During the early and late steps of infection with the Gram-positive bacterium B. anthracis, the tripartite anthrax toxin is secreted as major virulence factor in order to kill host immune cells such as macrophages or neutrophils. Like other AB-type toxins, it is composed of a surface binding/translocation moiety, the protective antigen (PA, 83 kDa), and two cytotoxic subunits, lethal factor (LF, 90 kDa) and edema factor (EF, 93 kDa). After cleavage by furin-like proteases, the truncated 63 kDa-sized PA monomer oligomerizes either into homo-heptamers (PA7) or homo-octamers (PA8). While PA8 can bind up to four factors, only three of them can simultaneously bind to PA7. Both enzymatic substrates bind to the upper rim of the PA oligomer via their N-terminal domains in a competitive manner.

We determined three structures of the fully-loaded heptameric anthrax lethal toxin complex, which differ in the position and conformations of the bound LFs. Due to a symmetry mismatch, three LFs occupy six binding sites of the heptameric PA7 complex, leaving one PA site empty. Binding of LF to a single PA protomer is mediated via the N-terminal domain of LF, orienting its bulky C-terminal domain such that the adjacent PA protomer is not accessible for binding. In this way a single lethal factor de facto occupies two of the seven binding sites of PA7. In the chain of LFs, the C-terminal domain of the anterior LF binds to the N-terminal domain of the following one, creating a directionality in the complex. Consequently, if two LFs are bound, three free PA binding sites are available, of which only two can potentially be occupied due to steric clashes. This results in the two complexes PA7LF2+1A and PA7LF2+1B, that differ in the binding position of the third LF. In two of our structures, PA7LF2+1A and PA7LF2+1B, two LFs only interact at one position which is located next to the major LF-PA interface. However, we only found that the N-terminal region of one LF (2LF) resides in the α-clamp, adopting the “open” conformation as described for PA8LF4. In the other LFs (1LF, 3LF), this region is flexible and not interacting with the α-clamp.

>[7x]MGHHHHHHHHHHSSGHIDDDDKHMEVKQENRLLNESESSSQGLLGYYFSDLNFQAPMVVTSSTTGDLSIPSSELENIPSENQYFQSAIWSGFIKVKKSDEYTFATSADNHVTMWVDDQEVINKASNSNKIRLEKGRLYQIKIQYQRENPTEKGLDFKLYWTDSQNKKEVISSDNLQLPELKQKSSNSRKKRSTSAGPTVPDRDNDGIPDSLEVEGYTVDVKNKRTFLSPWISNIHEKKGLTKYKSSPEKWSTASDPYSDFEKVTGRIDKNVSPEARHPLVAAYPIVHVDMENIILSKNEDQSTQNTDSQTRTISKNTSTSRTHTSEVHGNAEVHASFFDIGGSVSAGFSNSNSSTVAIDHSLSLAGERTWAETMGLNTADTARLNANIRYVNTGTAPIYNVLPTTSLVLGKNQTLATIKAKENQLSQILAPNNYYPSKNLAPIALNAQDDFSSTPITMNYNQFLELEKTKQLRLDTDQVYGNIATYNFENGRVRVDTGSNWSEVLPQIQETTARIIFNGKDLNLVERRIAAVNPSDPLETTKPDMTLKEALKIAFGFNEPNGNLQYQGKDITEFDFNFDQQTSQNIKNQLAELNATNIYTVLDKIKLNAKMNILIRDKRFHYDRNNIAVGADESVVKEAHREVINSSTEGLLLNIDKDIRKILSGYIVEIEDTEGLKEVINDRYDMLNISSLRQDGKTFIDFKKYNDKLPLYISNPNYKVNVYAVTKENTIINPSENGDTSTNGIKKILIFSKKGYEIG;>[3x]MNIKKEFIKVISMSCLVTAITLSGPVFIPLVQGAGGHGDVGMHVKEKEKNKDENKRKDEERNKTQEEHLKEIMKHIVKIEVKGEEAVKKEAAEKLLEKVPSDVLEMYKAIGGKIYIVDGDITKHISLEALSEDKKKIKDIYGKDALLHEHYVYAKEGYEPVLVIQSSEDYVENTEKALNVYYEIGKILSRDILSKINQPYQKFLDVLNTIKNASDSDGQDLLFTNQLKEHPTDFSVEFLEQNSNEVQEVFAKAFAYYIEPQHRDVLQLYAPEAFNYMDKFNEQEINLSLEELKDQRMLARYEKWEKIKQHYQHWSDSLSEEGRGLLKKLQIPIEPKKDDIIHSLSQEEKELLKRIQIDSSDFLSTEEKEFLKKLQIDIRDSLSEEEKELLNRIQVDSSNPLSEKEKEFLKKLKLDIQPYDINQRLQDTGGLIDSPSINLDVRKQYKRDIQNIDALLHQSIGSTLYNKIYLYENMNINNLTATLGADLVDSTDNTKINRGIFNEFKKNFKYSISSNYMIVDINERPALDNERLKWRIQLSPDTRAGYLENGKLILQRNIGLEIKDVQIIKQSEKEYIRIDAKVVPKSKIDTKIQEAQLNINQEWNKALGLPKYTKLITFNVHNRYASNIVESAYLILNEWKNNIQSDLIKKVTNYLVDGNGRFVFTDITLPNIAEQYTHQDEIYEQVHSKGLYVPESRSILLHGPSKGVELRNDSEGFIHEFGHAVDDYAGYLLDKNQSDLVTNSKKFIDIFKEEGSNLTSYGRTNEAEFFAEAFRLMHSTDHAERLKVQKNAPKTFQFINDQIKFIINS>SNAQEQRMSHHYATIEVSQQLEQLLGDQLVILLRETPDGQALERSQNDFRRVLEQGRANTVDSAEQAALDGVRDAYLQLQAHTPALLEAPMADNDGF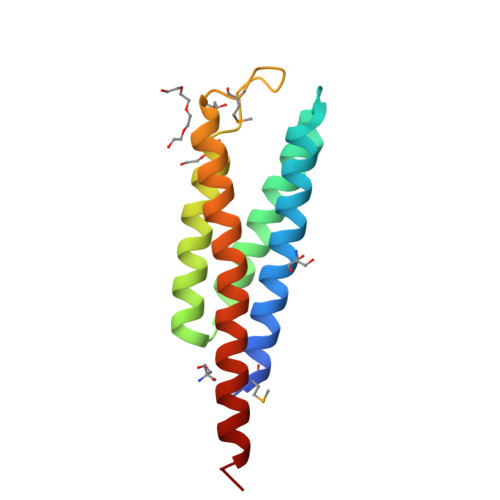SEAFNGLRLRLQDLQQLALAGISEAETSARHRA[2x]>[6x]PEKSLYEMAVEQFNRAASLMDLESDLAEVLRRPKRVLIVEFPVRMDDGHVEVFTGYRVQHNVARGPA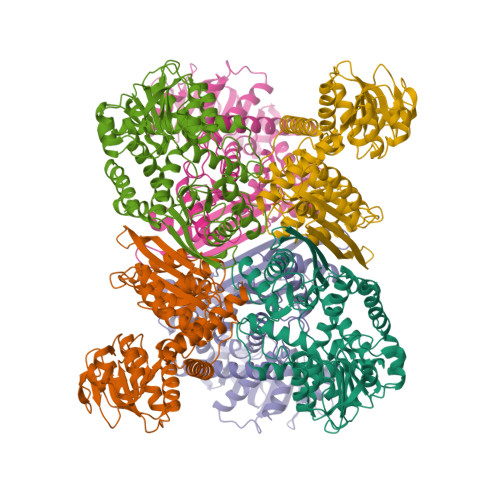KGGIRYHPDVTLDEVKALAFWMTWKTAVMDLPFGGGKGGVRVDPKKLSRNELERLSRRFFSEIQVIIGPYNDIPAPDVNTNADVIAWYMDTYSMNVGHTVLGIVTGKPVELGGSKGREEATGRGVKVCAGLAMDVLGIDPKKATVAVQGFGNVGQFAALLISQELGSKVVAVSDSRGGIYNPEGFDVEELIRYKKEHGTVVTYPKGERITNEELLELDVDILVPAALEGAIHAGNAERIKAKAVVEGANGPTTPEADEILSRRGILVVPDILANAGGVTVSYFEWVQDLQSFFWDLDQVRNALEKMMKKAFNDVMKVKEKYNVDMRTAAYILAIDRVAYATKKRGIYP> NLYQFKNMIQCTVPSRSWADFADYGCYCGKGGSGTPVDDLDRCCQTHDNCYNEAENISGCRPYFKTYSYECTQGTLTCKGDNNACAASVCDCDRLAAICFAGAPYN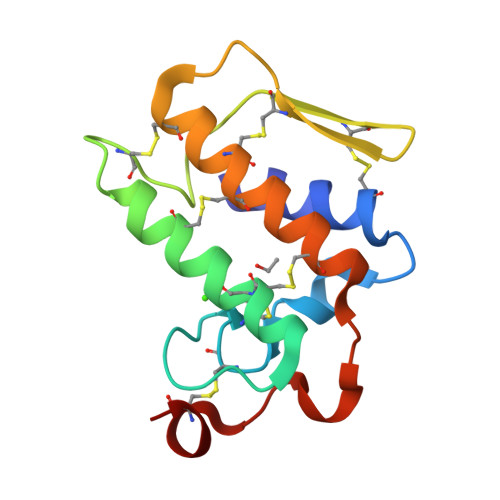DANYNIDLKARCN>[2x]MHHHHHHSSGRENLYFQGETSVPPGSALVGPSCVMDDFRDPQRWKECAKQGKMPCYFDLIEENVYLTERKKNKSHRDIKRMQCECTPLSK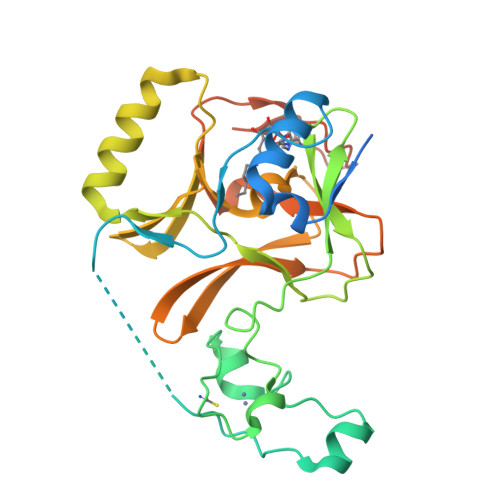DERAQGEIACGEDCLNRLLMIECSSRCPNGDYCSNRRFQRKQHADVEVILTEKKGWGLRAAKDLPSNTFVLEYCGEVLDHKEFKARVKEYARNKNIHYYFMALKNDEIIDATQKGNCSRFMNHSCEPNCETQKWTVNGQLRVGFFTTKLVPSGSELTFDYQFQRYGKEAQKCFCGSANCRGYLGGENRVSIRAAGGKMKKERSRK>METHTFGTFQDAYLSQLRDIYHSPEFRNAPRGQASRERIGAGFRLLDPVQRHISVPARRANVVFNFAEALWYLSGSDRLDFIQYYAPGIAAYSADGRTLRGTAYGPRIFRHPAGGVNQWENVVKTLTDDPDSKRAVIQIFDPRELAVADNIDVACTLALQFLIRDGLLCGIGYMRANDAFRGAVSDVFSFTFLQEFTARYLGLGIGTYHHVVGSVHIYDSDARWAERVLDAATPDGGPRPGFPAMPDGDNWPHVRRVLEWEERLRTNAARLSADALDALDLPAYWKHVVALFEAHRQVRHEDTPDRALLAALPEVYRQSLAVKWPGHFGSPAG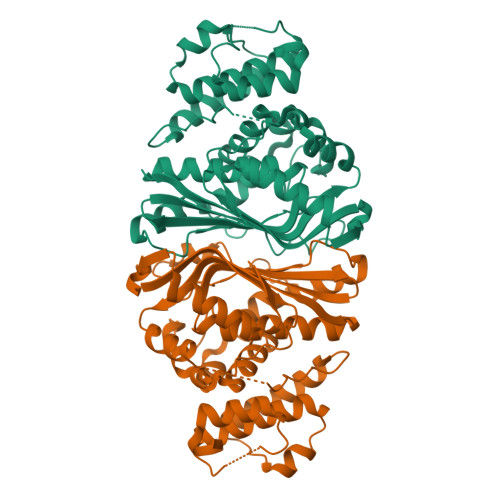SLEHHHHHH[2x]>[4x]GKVGDRPIEQQLALGYIKALTEHDYQTLSKYYNRDSVFYDKTADTKYIGTRSIIAFLQRSHEGVLE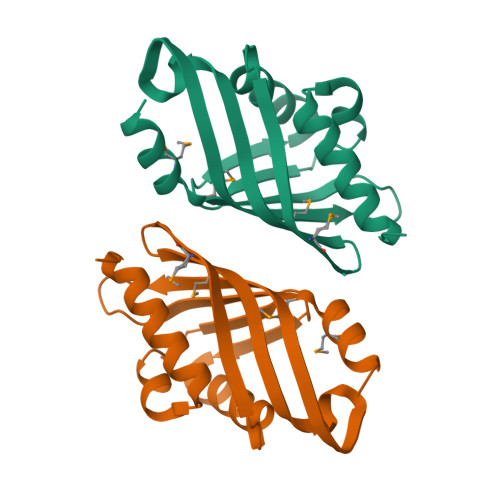FDFNIEHMFNTGPLVVMIGNYHLRGPGEQFGKPGKIIDIAIPGVTTLKFDPNTQRLTEQVDLMDYQTMSDQLQSQ>GPGSELPQMVQQLNSPDQQELQSALRKLSQIASGGNEQIQAVIDAGALPALVQLLSSPNEQILQEALWALSNIASGGNEQIQAVIDAGALPALVQLLSSPNEQILQEALWALSNIASGGNEQIQAVIDAGALPALVQLLSSPNEQILQEALWALSNIASGGNEQIQAVIDAGALPALVQLLSSPNEQILQEALWALSNIASGGNEQIQAVIDAGALPALVQLLSSPNEQILQEALWALSNIASGGNEQKQAVKEAGALEKLEQLQSHENEKIQKEAQEALEKLQSH[4x];> RRRR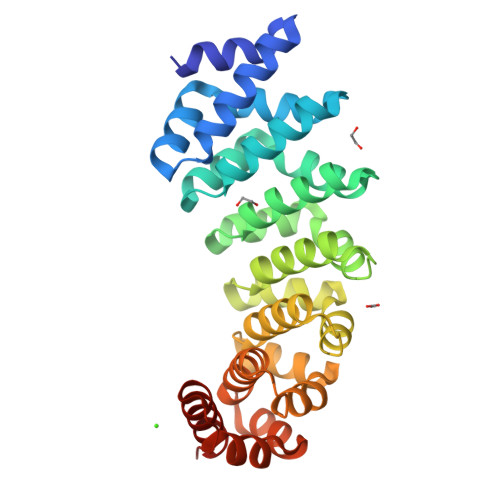RRRR>MRLELPVIPLRNTVILPHTTTPVDVGRAKSKRAVEEAMGADRLIFLVAQRDPEVDDPAPDDLYTWGVQAVVKQAMRLPDGTLQVMVEARARAQVTDYIPGPYLRARGEVFSEIFPIDEAVVRVLVEELKEAFEKYVANHKSLRLDRYQLEAVKGTSDPAMLADTIAYHATWTVAEKQEILELTDLEARLKKVLGLLSRDLERFELDKRVAQRVKEQMDTNQREYYLREQMKAIQKELGGEDGLSDLEALRKKIEEVGMPEAVKTKALKELDRLERMQQGSPEATVARTYLDWLTEVPWSKADPEVLDINHTRQVLDEDHYGLKDVKERILEYLAVRQLTQGLDVRNKAPILVLVGPPGVGKTSLGRSIARSMNRKFHRISLGGVRDEAEIRGHRRTYIGAMPGKLIHAMKQVGVINPVILLDEIDKMSSDWRGDPASAMLEVLDPEQNNTFTDHYLDVPYDLSKVFFITTANTLQTIPRPLLDRMEVIEIPGYTNMEKQAIARQYLWPKQVRESGMEGRIEVTDAAILRVISEYTREAGVRGLERELGKIARKGAKFWLEGAWEGLRTIDASDIPTYLGIPRYRPDK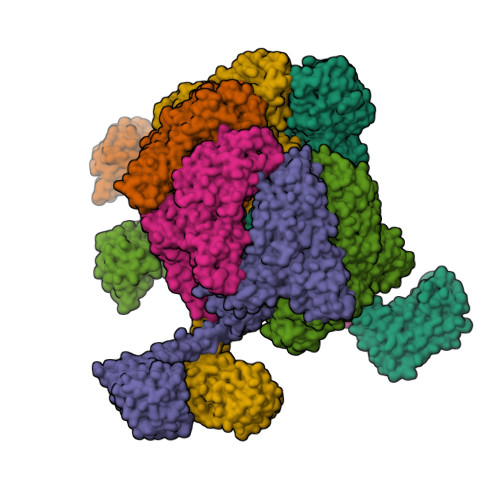AETEPQVGTAQGLAWTPVGGTLLTIEVAAVPGSGKLSLTGQLGEVMKESAQAALTYLRAHTQDYGLPEDFYNKVDLHVHVPDGATPKDGPSAGITMATAIASALSRRPARMDIAMTGEVSLRGKVMPIGGVKEKLLAAHQAGIHKIVLPKDNEAQLEELPKEVLEGLEIKLVEDVGEVLEYLLLPEPTMPPVVQPSDNRQQPGAGA[6x]>MDAATTRVGLTDLTFRLLRESFADAVSWVAKNLPARPAVPVLSGVLLTGSDNGLTISGFDYEVSAEAQVGAEIVSPGSVLVSGRLLSDITRALPNKPVDVHVEGNRVALTCGNARFSLPTMPVEDYPTLPTLPEETGLLPAELFAEAISQVAIAAGRDDTLPMLTGIRVEILGETVVLAATDRFRLAVRELKWSASSPDIEAAVLVPAKTLAEAAKAGIGGSDVRLSLGTGPGVGKDGLLGISGNGKRSTTRLLDAEFPKFRQLLPTEHTAVATMDVAELIEAIKLVALVADRGAQVRMEFADGSVRLSAGADDVGRAEEDLVVDYAGEPL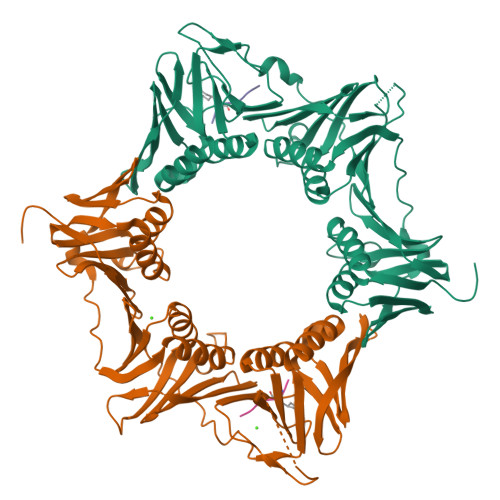TIAFNPTYLTDGLSSLRSERVSFGFTTAGKSALLRPVSGDDRPVAGLNGNGPFPAVSTDYVYLLMPVRLPG[4x];>XQADLF[4x]> GSSKLIHVPKEDNSKEVTLDSLLEEGVLDKEIHKAITRMEFPGLTPVQQKTIKPILSSEDH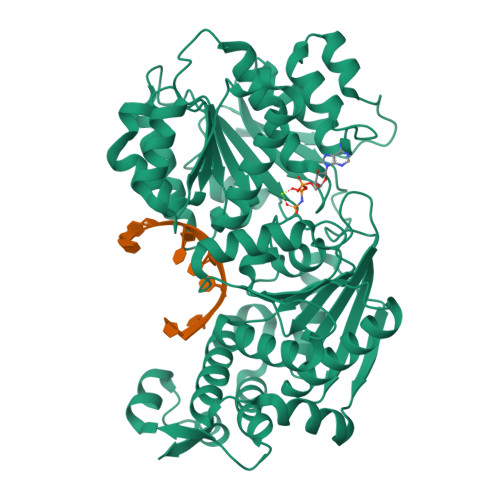DVIARAKTGTGKTFAFLIPIFQHLINTKFDSQYMVKAVIVAPTRDLALQIEAEVKKIHDMNYGLKKYACVSLVGGTDFRAAMNKMNKLRPNIVIATPGRLIDVLEKYSNKFFRFVDYKVLDEADRLLEIGFRDDLETISGILNEKNSKSADNIKTLLFSATLDDKVQKLANNIMNKKECLFLDTVDKNEPEAHERIDQSVVISEKFANSIFAAVEHIKKQIKERDSNYKAIIFAPTVKFTSFLCSILKNEFKKDLPILEFHGKITQNKRTSLVKRFKKDESGILVCTDVGARGMDFPNVHEVLQIGVPSELANYIHRIGRTARSGKEGSSVLFICKDELPFVRELEDAKNIVIAKQEKYEPSEEIKSEVLEAVTEEPEDISDIVISLISSYRSCIKEYRFSERRILPEIASTYGVLLNDPQLKIPVSRRFLDKLGLSRSPIGKAMFEIRDYSSRDGNNKSYDYDDDSEISFRGNKNYNNRSQNRDYDDEPFRRSNNNRRSFSRSNDKNNYSSRNSNIY> GAMEAMQKNELNSKIPIIFGLINSYQIHNLLEQHNAKTKESKAVFLIRDSSTYPGLLTISYYCQEQDIVKHIRFGLTDKGWKTAPKPPHEPLKSDSPEI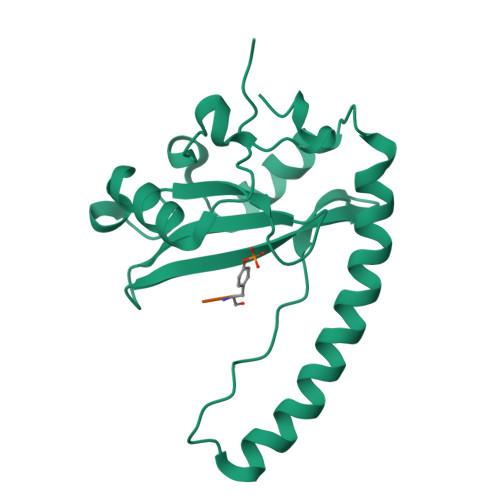KEKYTLDKIKFERKMKQFINTAKKLFEQHIRAESFKTLIMELKIHEFNLEGLIKPTRSQASQEKHFTDYV;> HYNGEAYEDDEHH>[3x]GMKNEVFFGEGMKVVAAAYPDLYDI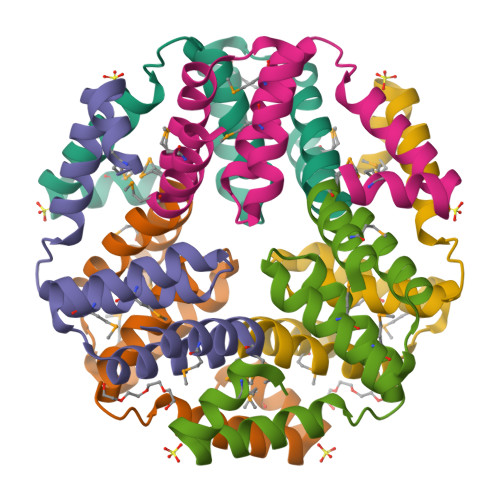IVKLNDTVFTGKTLDYKTQKLIAIGIVASRCDEVAIEKQMKSAMKELGITKEEIADVLRVVLLTSGMPAFTKAMKILEKL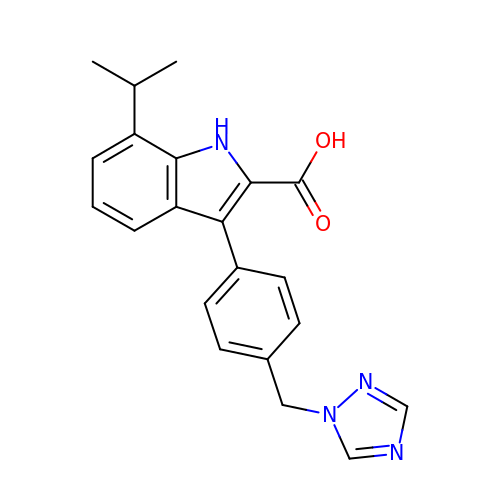7-propan-2-yl-3-[4-(1,2,4-triazol-1-ylmethyl)phenyl]-1~{H}-indole-2-carboxylic acid | C21 H20 N4 O2 | PWOCNZSEEMMUEH-UHFFFAOYSA-N> MDRKTRLSEPPTLALRLKPYKTAIQQLRSVIRALKENTTVTFLPTPSLILQTVRSHCVSKITFNSSCLYITDKSFQPKTINNSTPLLGNFMYLTSSKDLTKFYVQDISDLSAKISMCAPDFNMEFSSACVHGQDIVRESENSAVHVDLDFGVVADLLKWIGPHTRVKRNVKKAPCPTGTVQILVHAGPPAIKFILTNGSELEFTSNNRVSFHGVKNMRINVQLKNFYQTLLNCAVTKLPCTLRIVTEHDTLLYVASRNGLFAVENFLTEEP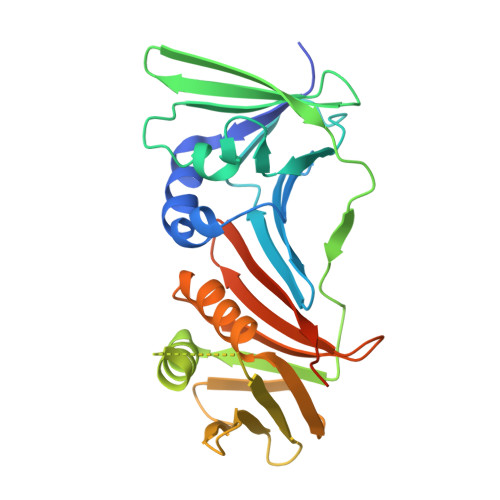FQRGDPFDKNYVGNSGKSR>GSKGRLVIYCSATNVMCENAAKTFEQKYDVKTSFIRNGSGSTFAKIEAEKNNPQADVWYGGTLDPQSQAGELGLLEAYRSPNIDQIMPKFQDPAKVKGNLSSAVYIGILGFAVNTERLKKLGIEKIPQCWNDLTDPKLKGEIQIADPQSSGTAYTAIATFAQLWGEDKAFDYFKHLHPNISQYTKSGITPARNAARGETTVGIGFLHDYALEKEQGAPLEMVVPCEGTGYELGGVSILKGARNLDNAKLFVDFALSKEGQETAWKKGQALQTLTNTTAEQSPLAFDLTKLKLIDYDFEKYGASDERKRLINKWVDEIKLAK[2x]

In this study, we investigate AfuABC (Actinobacillus ferric uptake ABC), a BPDT originally identified as an iron-specific transporter in Actinobacillus pleuropneumoniae, a Gram-negative upper respiratory tract pathogen. The locus afuABC encodes 3 polypeptides corresponding to a conventional BPDT–AfuA (a periplasmic binding protein or PBP), AfuB (an inner membrane permease), and AfuC (a cytosolic ATPase). AfuA is a class II/cluster D periplasmic binding protein with two globular α/β domains linked by a dual β-stranded hinge. Instead, AfuABC is a trio of proteins that bind and transport sugar-phosphates such as glucose-6-phosphate (G6P).

To structurally characterize the ligand of AfuA, a 1.6Å crystal structure of ligand-bound A. pleuropneumoniae AfuA purified from E. coli was solved by use of sulfur single wavelength anomalous diffraction. In the binding cleft, we unexpectedly observed positive electron density and identified glucose-6-phosphate (β-G6P) as the bound ligand with a small (~5%) portion of density at carbon 2 corresponding to mannose-6-phosphate (β-M6P). In the binding cleft, His205, Asp206 and Glu229 interact multivalently with the sugar ring while Ser37 and Thr150 form hydrogen bonds with the phosphate moiety of G6P. Isothermal titration calorimetry (ITC) validated the binding affinity of A. pleuropneumoniae AfuA for β-G6P at 24 nM with favourable values of enthalpy and entropy change. The mutations T150A and S37A lowered but did not eliminate binding to G6P, whereas mutations to the sugar-binding residues (H205A, D206A and E229A) completely abrogated the interaction. This indicates that the hydrogen-bonding capacity of the sugar-coordinating residues is the critical determinant in mediating binding of potential sugar phosphates. In AfuA, the essential residues His205 and Asp206 form multivalent hydrogen bonds to the sugar moiety of ligands and function as the primary determinants of ligand selectivity. On the opposing end of the pocket, redundant phosphate-coordinating residues such as Ser37 cooperate to hold the phosphate moiety of ligands. The structures shown here are the first structural data for a non-enzymatic sugar-phosphate (i.e. G6P) binding protein.>[2x]ETGFDIGLSTKCVTIPTEMAMCNDVGYSEMRLPNLMGHTNMAEVVPKSAEWQNLLQTGCHPYARTFLCSLFAPVCLDTFIQPCRS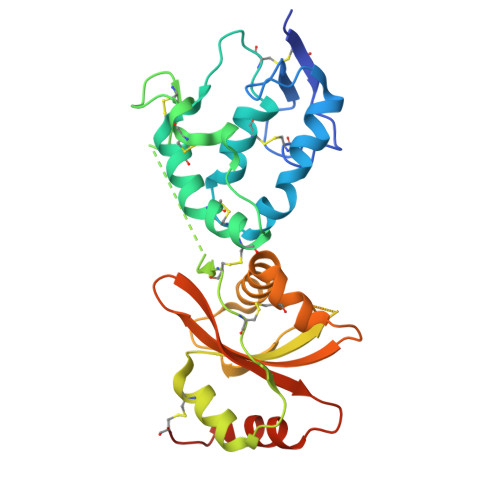MCVAVRDSCAPVLACHGHSWPESLDCDRFPAGEDMCLDTLSKEYQYSYKELPKPSCQGCPLIEEFFSHKTVLEAFCDNNFAVKVKLAKKKSASGLYEYETEGPVEFIKQGLLLPYDTRTMIEQWLLINENCAQKLIRTRPTVYVIAGDIHHGKVKVNRIFHWQKKDSQLTLATRRWRHHKCGTKHHHHHH> MIDLREDTWTLQLYAQRYKGLSPKNSRELQLRMEYDPLKPNLPTSGEEQNSKPEWLNTPPCLIPESESLDKAKGALVGLAIGDAIGTTLEFLPRDKLHVNDMVGGGPFRLQPGEWTDDTSMALCLAESYISAGRLDITLFREKLVRWYRHGENSSNGRCFDIGNTTRNALEQYLKHGASWFGNTEPETAGNAAIIRQAPTSIFRRKSLQRTFADSDSQSMATHCAPESMASCQFLGFILNYLINGSSREKAFSPHVMPLPVRVLLINAGEYKEKKRDEIRSSGYVIDTLEAAMWAVWNTDNFHDAILLAANLGDDADSVAATTGQIAGALYGYSNIPKPWLDKLVQQERISNLAEQLFYMAPEEDF;> GQEQAKVWTQTARANAEKNNAQLSTLLTDDQIGAIYGYTTNEGYTALNPALRGQTPLTPELEAFTGHVTDGLNKLPAYNGETYRGTTLPAHILEQNQIGGTVS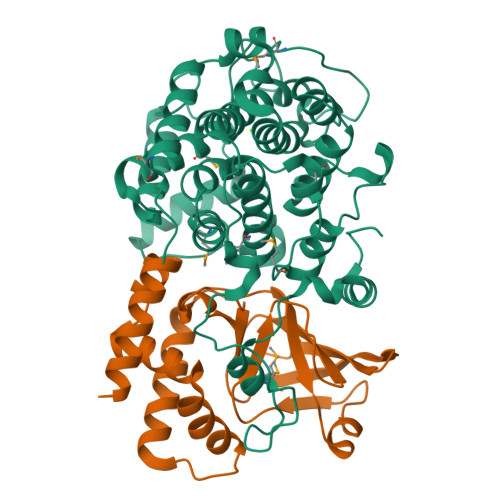DGGFMSTSAKTPFDGDVSISVRGNSGKQIDFLSKYKNEAEVLYPPNTRFEVINRIEQNGTTHLLYREIP>[4x]GACACCUGAUUC;>G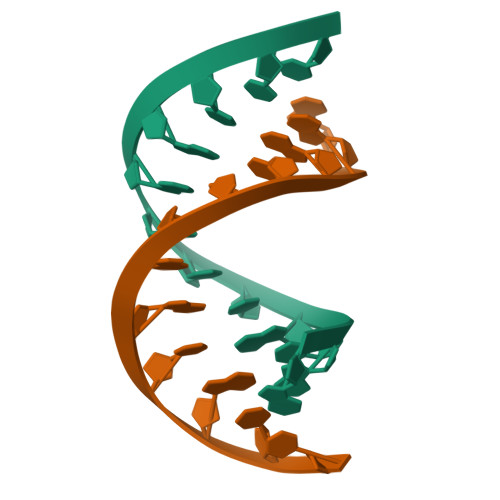AATCAGGTGTC[4x]(phenylmethyl) 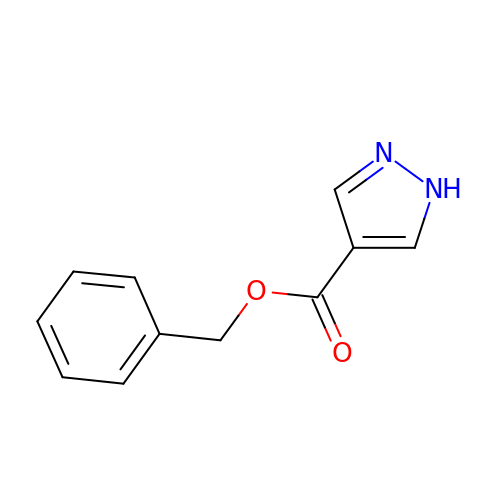1~{H}-pyrazole-4-carboxylate | C11 H10 N2 O2 | OZQCSFKTURXPAA-UHFFFAOYSA-N> AQEVTGMVFQPFSEVQGELSTVTQAPVTDSYARVEYHIECEAAINEQINIEYTISYVYHALHSYFARDNVGLPGFAKFFKEASDEEREHAHMLMDYQTKRGGRVELKPLAAPEMEFANDDKGEALYAMELALSLEKLNFQKLQALQ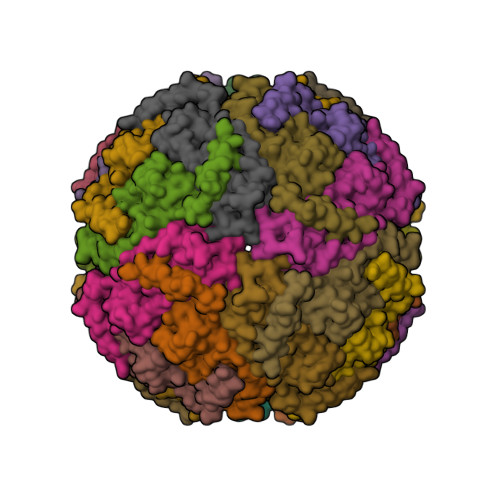AIADKHKDAALCDFVEGGLLSEQVDAVKEHAVYVSQLRRVGKGVGVYLLDQELGEEEA> KHSCIAVIDAGSTGSRLHIYSYDTDDTNTPIHIEEIWNKKIKPGFAS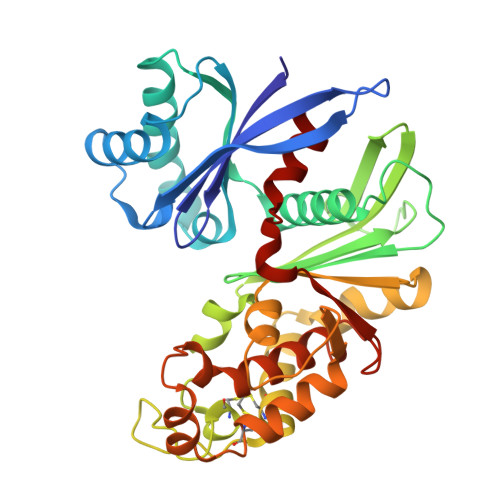IQPNSVTIDAYLTMLLADAPIHNIPVYFYATAGMRLLPQSQQKKYYDELEYWFRQQSQWQLVEAKTITGNDEALFDWLAVNYKLDTLKSVQNKSVGVMDMGGASVQIVFPMPKNAEISKHNQVELNIYGQNINLYVHSFLGLGQTEMSHQFLNSPSCFANDYPLPDGESGQGNAPSCKEEVTSLMNSVHKVNQQIQPLLALNPVNEWYSIGGISNLASSQLFHFENSELTNQSLLQQGDNQICHQQWDILNGQYPDDEYLYQYCLLSSYYYALMVDGYGINPNQTIHYIPPEQNLDWTIGVVLHRA TOLRESTAT | C16 H14 F3 N O3 S | 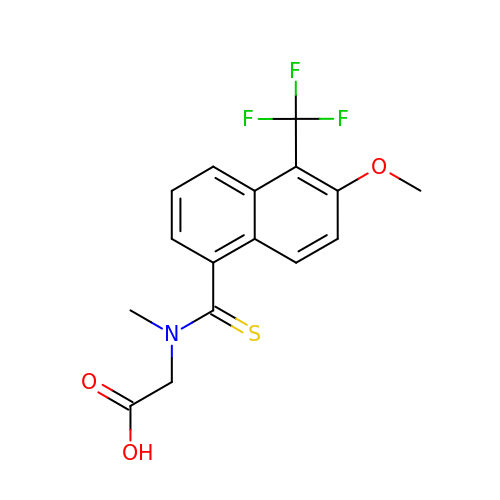LUBHDINQXIHVLS-UHFFFAOYSA-N In phylogenetically diverse bacteria, the conserved protein RapZ plays a central role in RNA-mediated regulation of amino-sugar metabolism. RapZ contributes to the control of glucosamine phosphate biogenesis by selectively presenting the regulatory small RNA GlmZ to the essential ribonuclease RNase E for inactivation. Here, we report the crystal structures of full length Escherichia coli RapZ at 3.40 Å and 3.25 Å, and its isolated C-terminal domain at 1.17 Å resolution. The structural data confirm that the N-terminal domain of RapZ possesses a kinase fold, whereas the C-terminal domain bears closest homology to a subdomain of 6-phosphofructokinase, an important enzyme in the glycolytic pathway.

Using limited proteolysis, the C-terminal half of RapZ (encompassing residues 154–284) was identified as a domain that could withstand digestion. Analysis by SEC-MALS (size-exclusion chromatography with multi-angle light scattering) and AUC (analytical ultracentrifugation) indicate that in isolation this protein domain is a homodimer. Well-ordered crystals were obtained of the purified RapZ-CTD, and a native dataset from a single crystal was collected at 1.17 Å resolution. Overall, the electron density was readily interpretable and allowed residues 156–281 to be modelled. The protein forms a crystallographic dimer with a symmetry-related copy, burying 1051.5 Å2 of solvent accessible surface area as determined by PISA analysis. This self-interacting interface is likely to account for the stable homodimer observed in solution. Of note are a cluster of basic residues around an extended loop on the surface of RapZ-CTD, including arginine 196 and lysines 251 and 281. During the process of modelling and refinement, clearly defined electron density for a non-protein ligand was observed in a pocket composed of the side chains of residues His190, His252, Arg253 and the backbone of Thr248 and Gly249. During optimization of the protein crystals, we found the addition of malonate to be extremely beneficial for crystal growth, and a malonate molecule accounts for this density excellently. RapZ-CTD unexpectedly exhibits distant structural homology to the fructose-6-phosphate binding domain of PFK, suggesting a common evolutionary origin.

> GKRERELTMVFESFGFKHGIPIDADYVFDVRFLPNPHWDPKLRPMTGLDKPVAAFLDRHTEVHNFIYQTRSYLELWLPMLETNNRSYLTVAIGCTGGKHRSVYIAEQLADYFRSRGKNVQSRHRTLEKRKP The gene of ETAE_2186 was among the top 3 upregulated genes and was annotated as a hypothetical thioredoxin; here, we named it Trx-like protein (Trxlp). In this study, we found that one of the most significant infection-induced E. piscicida genes, trxlp, could be secreted and translocated into the cytosol of host cells upon infection, showing a conserved crystal structure to the host thioredoxin protein. Furthermore, Trxlp could mimic endogenous TRX1 to directly target the TRX-binding domain of ASK1 (ASK1-TBD) and inhibit its activation, subsequently suppressing Erk/p38-MAPK signaling, correlating to limit bacterial virulence and replication in vivo. Taken together, our results provide the first comprehensive, functional analysis of the E. piscicida Trx family protein Trxlp, a novel virulence effector that mimics endogenous TRX1 to target ASK1 and suppress its activation, thereby inhibiting the phosphorylation of Erk1/2- and p38-MAPKs and disrupting the expression of inflammatory cytokines and diminishing the host antibacterial defense.

The structure was refined to an R-value of 17.7% (Rfree = 21.5%) with good geometry at a resolution of 1.98 Å. Trxlp displays a similar structure to that of the canonical Trx fold, consisting of a β1-α1-β2-α2-β3-α3-β4-β5-α4 topology. Trxlp contains a central β-sheet composed of 3 parallel (β1, β2, β3) and 2 antiparallel strands (β4, β5). This central β-sheet is sandwiched by 2 layers of helices: a bottom layer with 2 helices (α1, α3) and a top layer with the other 2 helices (α2, α4). The structure obtained here is in reduced form, as evidence by the 3.3 Å distance between 2 sulfur atoms of 2 cysteines in the CXXC motif. Trxlp can be superimposed to Trxs from other species, with root-main-square deviation (rmsd) values ranging from 1.54 to 1.74 Å for around 100 equivalent Cα pairs. Minor conformational differences among these structures were observed in flexible loop regions connecting α helices and β strands. Trxlp shares a conserved structure and critical WCXXC-motif site not only with bacterial Trxs, but also with mammalian Trxs. Notably, either mutation in Trxlp (W50F, C51/53S, FSXXS) or mutation in ASK1-TBD (C250S) significantly impaired the interactions between them. Taken together, unlike the classical Trxs, Trxlp might not exhibit robust redox activity.

> SVEPYSDAAFTQAQASGAPVLVDVYADWCPVCKRQERELTPLFAQPAQRDLRVFKVNFDTQKAALQQFRVSQQSTLILYRNGQEVRRSIGETSPSALSDFLTR3-(4,5-diphenyl-1,3-oxazol-2-yl)propanoic acid | C18 H15 N O3 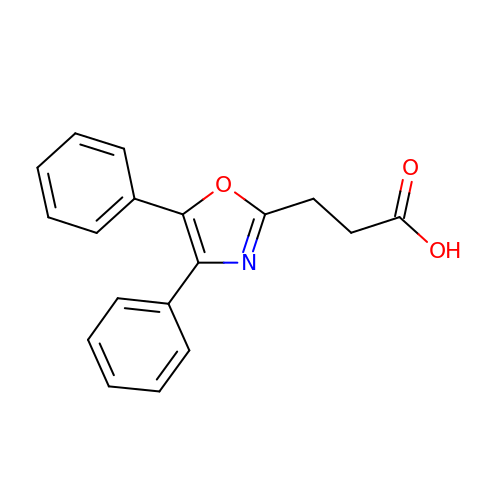| OFPXSFXSNFPTHF-UHFFFAOYSA-N> GLVPRGSHMFIMIGERINGMFKDIREAILNKDPRPIQEWARRQAEKGAHYLDVNTGP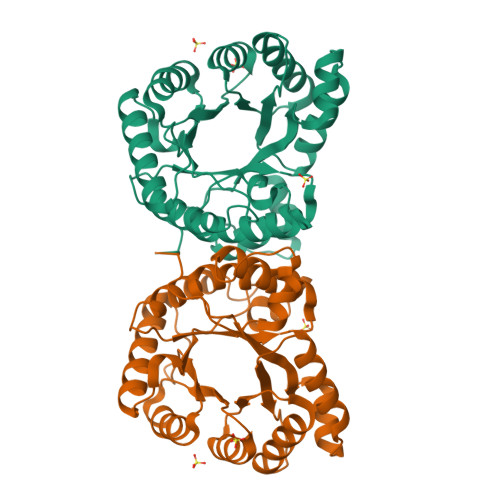TADDPVRVMEWLVKTIQEVVDLPCCLDSTNPDAIEAGLKVHRGHAMINSTSADQWKMDIFFPMAKKYEAAIIGLTMNEKGVPKDANDRSQLAMELVANADAHGIPMTELYIDPLILPVNVAQEHAVEVLETIRQIKLMANPAPRTVLGLSNVSQKCPDRPLINRTYLVMAMTAGLDAAIMDVDDDALVDAAATAHILLNKEIYCDSYLKTFRQK>[2x]MKVFREYI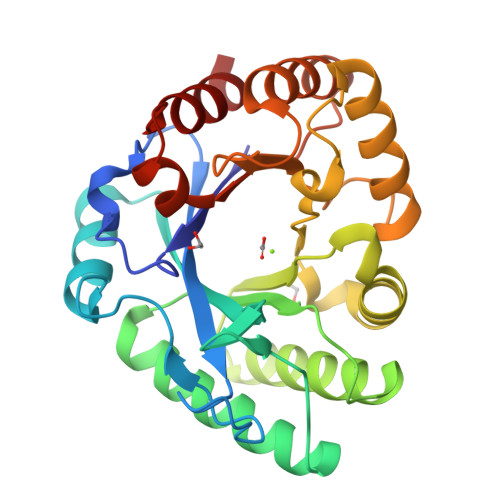GALYNGVQFTDVPINSGVTFHFILAFAIDYTSAAAATNGVFNIYWQNSVLTPAAVQAIKAQHSNVKVMVSLGGDTISGSPVQFTATSVSSWVANAVSSLTSLINQYHLDGIDIDYEHFDQVSTSTFVSCIGQLITQLKANNVISVASIAPFDGVESQYTALFGQYSSVIDLVNFQFYSYGAGTSASQYVSLYNTAASKYGGGAKVLASFSTGGVGPAPSTVLSACQQLKSSGTLPGIFIFSADGSYASSAKFQYEQQAQTLLTS> MSSEPLEPNQDVIIPRSRDSLGRPVYKAQLTRTDNQSEKVALIRQTAPLPVIFIPGIMGTNLRNKADKSEVWRPPNGLWPMDDLFASIGALWTWAWRGPKARQELLKAEQVEVDDQGTIDVGQSGLSEEAARLRGWGKVMRSAYNPVMGLMERRLDNIVSRRELQAWWNDEALSPPGDQGEEQGKVGPIDEEELLRASRYQFDVWCAGYNWLQSNRQSALDVRDYIENTVLPFYQKECGLDPEQMRRMKVILVTHSMGGLVARALTQLHGYERVLGVVHGVQPATGSSTIYHHMRCGYEGIAQVVLGRNAGEVTAIVANSAGALELAPSAEYREGRPWLFLCDAQGQVLKDIDGKPRAYPQNQDPYEEIYKNTTWYGLVPEQNSQYLDMSDKKEGLRVGPRDNFEDLIDSIANFHGELSAAGYHSETYAHYGADDSRHSWRDLIWKGDPTPLETPGATLNDDENGTYNSWFRRGLPTIVQGPLETGNPLDASG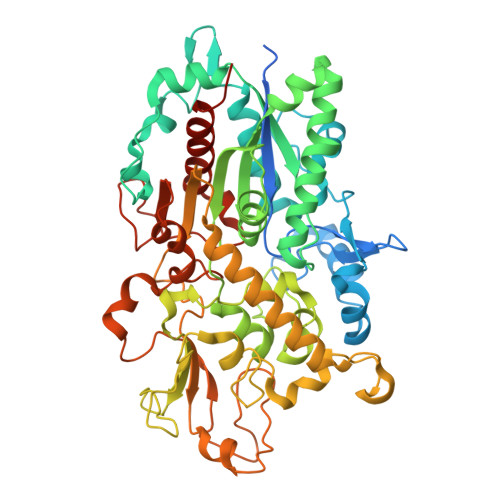SGGDETVPTDSGQAPALAGVKASFRHGSKGKGQANTKRGYEHQESYNDARAQWAALYGVIKITQLADWHPNDKGGT> MKNATFYLLDNDTTVDGLSAVEQLVCEIAAERWRSGKRVLIACEDEKQAYRLDEALWARPAESFVPHNLAGEGPRGGAPVEIAWPQKRSSSRRDI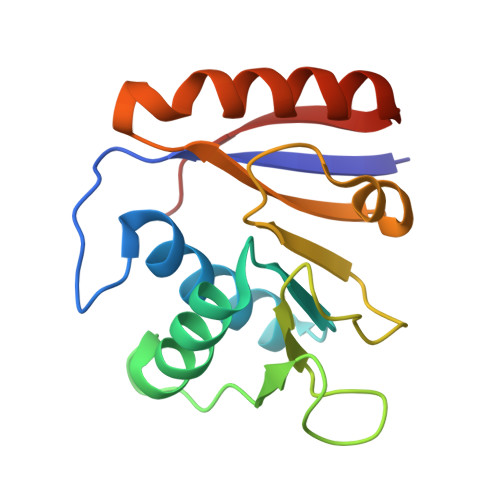LISLRTSFADFATAFTEVVDFVPYEDSLKQLARERYKAYRVAGFNLNTATWK> GGGGGGGG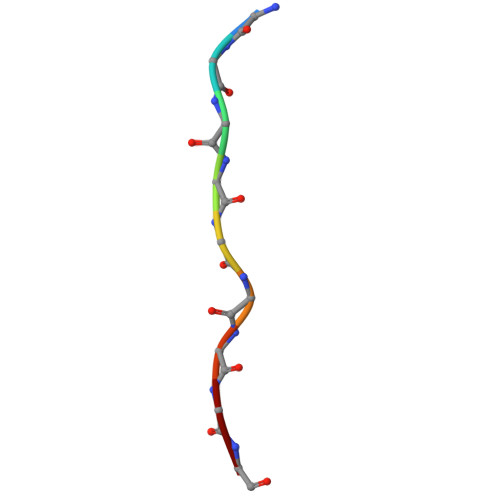G>[26x]MKKILNSLFSITLVMLVPFKVMASWYEVTGVATIVSSEETARLHALEDALFKAVNFSGADIGSISNLMPLLEESRNEYQFTNHEVRYILVESERKRRGKVEVKIRVDIYPSATGCHTDQYKKTILVGNIEVASPQQAVMGQIYQVGDDFSRVVNRQLDQTSRSFVSVGTTDYSISSNYPARTQMIAQDNGAQYIIGGVITDLTATVESQLLQDDIINRQFALEMKVFDGKTGHEVFNKAYREVARWPFAKTSQVDTRSARFWASTYGEMMLRVSRNIMLDLESELSCKITLPEVVAVFGNTVTMDLGRMHGVKEGDKLQLWHTASFIDQNGLPRNKVSQSEITLTVSRIYEHEAELTIDQPNLASSVQIGDVMNKIL;>MKRICLLALIATMSGCAMLEPIETDEVTQATTVVDAVEGDKSKEESSGIVDTLRGRSDPVAGDPAWAPIHPKKKPEHYAAATGSLFSAEHITDLYDDSKPRGIGDIITVTLDETTSATKSANADLSKTNEAQMDPLQVGGEELQIGGKYNFSYDLNNSNSFAGDSSAKQSNSISGYITVEVIEVLANGNLVIRGEKWMTLNTGDEYIRLSGTIRPDDISFDNTIASNRVSNARIQYSGTGVQQDMQEPGFLARFFNVAL[26x];>MKKLLFIVATLILVGCQPLQQMRQDEILVAVGYASVSEQTGRTVEEKRVRAMRASKIDAYRELAEQVYGMRVSGRAELQDQRLGIESTTGAVDGVIRGAEVVRSYLVEDSYVTELRLDIRKMDKLRDYGEVQQVPEKRQQTLF[26x];>CAMLEPIETDEVT[26x];>[26x]MKKLLLILMSVALFSTAAQAARIKDVAQVAGVRSNQLVGYGLVSGLPGTGEANPFTEQSFAAMLQNFGIQMPPGTKPKIKNVAAVMVTAELPPFSKPGQQVDVTVSSIGSAKSLRGGTLLQTFL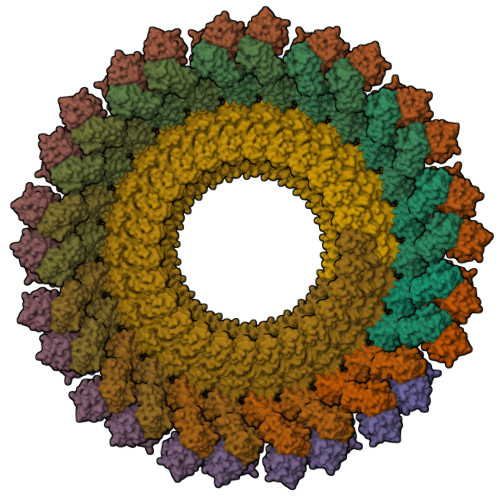KGLDGQVYAVAQGNLVVSGFSAEGADGSKIVGNNPTVGLISSGATVEREIPNPFGRGDYITFNLLESDFTTAQRMADAVNNFLGPQMASAVDATSVRVRAPRDVSQRVAFLSAIENLEFDPADGAAKIIVNSRTGTIVVGKHVRLKPAAVTHGGMTVAIKENLNVSQPNGFSGGQTVVVPDSDIEVSEEQGKMFKFEPGLTLDDLVRAVNQVGAAPSDLMAILQALKQAGAIEGQLIII;>[26x]MKKWLITSGVVFSLFSTSSFAVMGKRYVATPQQSQWEMVVNTPLECQLVHPIPSFGDAVFSSRANKKINLDFELKMRRPMGETRNVSLISMPPPWRPGEHADRITNLKFFKQFDGYVGGQTAWGILSELEKGRYPTFSYQDWQSRDQRIEVALSSVLFQNKYNAFSDCISNLLKYSFEDIAFTILHYERQGDQLTKASKKRLSQIADYIRHNQDIDLVLVATYTDSTDGKSASQSLSERRAESLRDYFQSLGLPEDRIQVQGYGKRRPIADNGSPIGKDKNRRVVISLGRTQV;>[26x]MKLRTVAASLLLTLVATTAKANVADVGAPVPIYTEAELIKLIEQNKHLQRVRADNCQLVEDIVARATRINLPAYEFLYGDMLAWGVCVEQDVELGLYYIENAAHQGLPAALEQIGRYYSRGTLVQQDKERAIPYLREAASMGNLNARIHLAELLLRDYGSPLDYEDAYRWLYNSVTADKRQHKRITVLRNGLEQRMPQNVIARAKRRDTFW>[4x]MDIKINDITLGNNSPFVLFGGINVLESLDSTLQTCAHYVEVTRKLGIPYIFKASFDKANRSSIH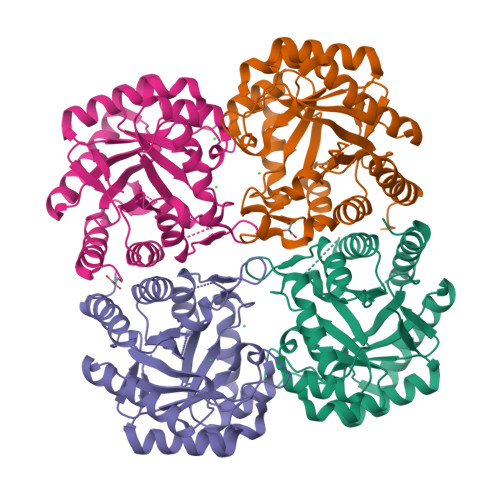SYRGVGLEEGLKIFEKVKAEFGIPVITDVHEPHQCQPVAEVCDVIQLPARLARQTDLVVAMAKTGNVVNIKKPQFLSPSQMKNIVEKFHEAGNGKLILCERGSSFGYDNLVVDMLGFGVMKQTCGNLPVIFDVTHSLQTRDAGSAASGGRRAQALDLALAGMATRLAGLFLESHPDPKLAKCDGPSALPLHLLEDFLIRIKALDDLIKSQPILTIE Recently, we identified and described a quinone reductase 2 (QR2) pathway in the brain, in which QR2 acts as a removable memory constraint and metabolic buffer within neurons. QR2 becomes overexpressed with age, and it is possibly a novel contributing factor to age-related metabolic stress and cognitive deficit. QR2 is a metabolic buffer, which becomes a metabolic stressor with age or when given certain substrates. We therefore created highly specific QR2 inhibitors (QR2is) to enable evaluation of chronic QR2 inhibition as a means to reduce biological age–related metabolic stress and cognitive decline.

To make QR2-ligand crystallization amenable, enable oral administration of the inhibitors, and eliminate undesirable formulations, HCl was conjugated to YB-537. Purified human QR2 (hQR2) was then cocrystalized in the presence of the water-soluble inhibitor. The resolved crystal structure of hQR2 in complex with YB-537 revealed that the protein exists as a homodimer, consistent with previous reports. YB-537 was found to bind to each monomer of the hQR2 homodimer, forming interactions with amino acids from both monomers as well as with the Flavin-adenine dinucleotide (FAD) cofactor. The plane of YB-537 stacks up parallel to the isoalloxazine ring of the FAD cofactor with an average distance of 3.5 Å between the planes of the two. YB-537 binds to the catalytic site through a series of hydrophobic and hydrogen bonds with both FAD and amino acids from both QR2 monomers. Specifically, YB-537 forms 6 contacts with G150, G151, and M155 and a hydrogen bond with N162 from one monomer (A-blue) and 8 contacts to F127, I129, F132, and F179 from the other monomer (B-red). Analysis of the SAR data revealed that the imidazo[1,2-a]pyridine heterocycles gave high activity of the sulfonamide and proved to be more potent compared with other heterocycles that were evaluated, forming crucial Pi-Pi interactions with the protein, attributing to its potency, as was later found in the resolved crystal structure. Specifically, while Asn162 in QR2, which is His162 in QR1, provides a hydrogen bond to plant YB-537 within the catalytic site and over the FAD prosthetic group, several other residues found only in QR2 also favorably interact electrostatically with the inhibitor. Further selectivity is likely caused by the 43aa C-terminus structure missing in QR2, which, in QR1, may physically hinder YB-537 inclusion to the catalytic site, as would residues within the QR1 catalytic site itself, such as Y127 and Y129.

>[2x]MAGLNDIFEAQKIEWHEMAGKKVLIVYAHQEPKSFNGSLKNVAVDELSRQGCTVTVSDLYAMNFEPRATDKDITGTLSNPEVFNYGVETHEAYKQRSLASDITDEQKKVREADLVIFQFPLYWFSVPAILKGWMDRVLCQGFAFDIPGFYDSGLLQGKLALLSVTTGGTAEMYTKTGVNGDSRYFLWPLQHGTLHFCGFKVLAPQISFAPEIASEEERKGMVAAWSQRLQTIWKEEPIPCTAHWHFGQ N-(2-ethoxyethyl)-N-{(2S)-2-hydroxy-3-[(5R)-2-(quinazolin-4-yl)-2,7-diazaspiro[4.5]dec-7-yl]propyl}-2,6-dimethylbenzenesulfonamide | C31 H43 N5 O4 S | 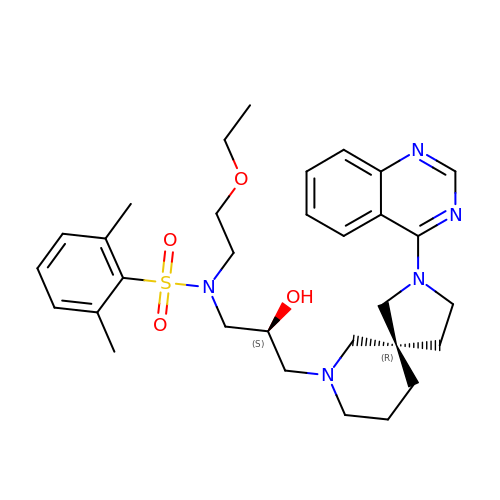ABPGHPHYGKUEIO-SUYBVONHSA-N> NPVENYIDEVLNEVLVVPNINSSNPTTSNSAPALDAAETGHTSSVQPEDVIETRYVQTSQTRDEMSLESFLGRSGCIHESKLEVTLANYNKENFTVWAINLQEMAQIRRKFELFTYTRFDSEITLVPCISALSQDIGHITMQYMYVPPGAPVPNSRDDYAWQSGTNASV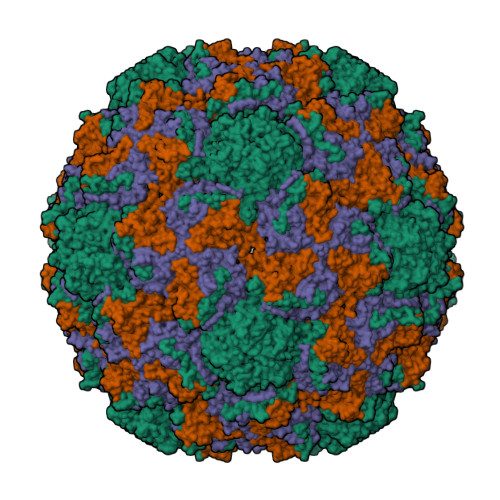FWQHGQAYPRFSLPFLSVASAYYMFYDGYDEQDQNYGTANTNNMGSLCSRIVTEKHIHKVHIMTRIYHKAKHVKAWCPRPPRALEYTRAHRTNFKIEDRSIQTAIVTRPIITTAGPSDMY;> SPTVEACGYSDRIIQITRGDSTITSQDVANAIVAYGVWPHYLSSKDASAIDKPSQPDTSSNRFYTLRSVTWSSSSKGWWWKLPDALKDMGIFGENMFYHYLGRSGYTIHVQCNASKFHQGTLIVALIPEHQIASALHGNVNVGYNYTHPGETGREVKAETRLNPDLQPTEEYWLNFDGTLLGNITIFPHQFINLRSNNSATIIAPYVNAVPMDSMRSHNNWSLVIIPICPLETSSAINTIPITISISPMCAEFSGARAKRQ;> GLPVFITPGSGQFLTTDDFQSPCALPWYHPTKEISIPGEVKNLVEICQVDSLVPINNTDTYINSENMYSVVLQSSINAPDKIFSIRTDVASQPLATTLIGEISSYFTHWTGSLRFSFMFCGTANTTVKLLLAYTPPGIAEPTTRKDAMLGTHVIWDVGLQSTISMVVPWISASHYRNTSPGRSTSGYITCWYQTRLVIPPQTPPTARLLCFVSGCKDFCLRMARDTNLHLQSGAIAQ>MASWSHPQFEKGGTHVAETSAPTRSEPDTRVLTLPGTASAPEFRLIDIDGLLNNRATTDVRDLGSGRLNAWGNSFPAAELPAPGSLITVAGIPFTWANAHARGDNIRCEGQVVDIPPGQYDWIYLLAASERRSEDTIWAHYDDGHADPLRVGISDFLDGTPAFGELSAFRTSRMHYPHHVQEGLPTTMWLTRVGMPRHGVARSLRLPRSVAMHVFALTLRTAAAVRLAEGA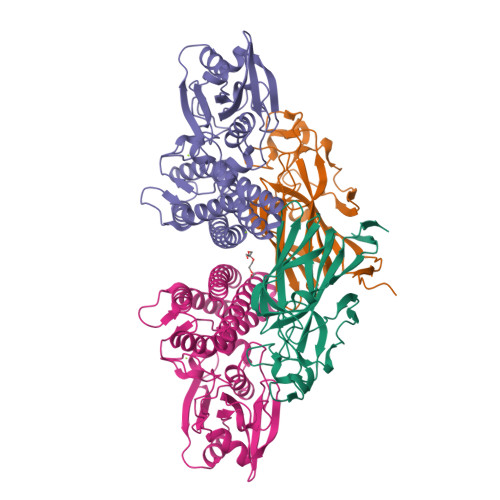TT[2x];>[2x]MGSSHHHHHHSQDPNSTTTAPPVELWTRDLGSCLHGTLATALIRDGHDPVTVLGAPWEFRRRPGAWSSEEYFFFAEPDSLAGRLALYHPFESTWHRSDGDGVDDLREALAAGVLPIAAVDNFHLPFRPAFHDVHAAHLLVVYRITETEVYVSDAQPPAFQGAIPLADFLASWGSLNPPDDADVFFSASPSGRRWLRTRMTGPVPEPDRHWVGRVIRENVARYRQEPPADTQTGLPGLRRYLDELCALTPGTNAASEALSELYVISWNIQAQSGLHAEFLRAHSVKWRIPELAEAAAGVDAVAHGWTGVRMTGAHSRVWQRHRPAELRGHATALVRRLEAALDLLELAADAVS> SKMDYDFKVKLSSERERVEDLFEYEGCKVGRGTYGHVYKAKRKDGKDDKDYALKQIEGTGISMSACREIALLRELKHPNVISLQKVFLSHADRKVWLLFDYAEHDLWHIIKFHRASKANKKPVQLPRGMVKSLLYQILDGIHYLHANWVLHRDLKPANILVMGEGPERGRVKIADMGFARLFNSPLKPLADLDPVVVTFWYRAPELLLGARHYTKAIDIWAIGCIFAELLTSEPIFHCRQEDIKTSNPYHHDQLDRIFNVMGFPADKDWEDIKKMPEHSTLMKDFRRNTYTNCSLIKYMEKHKVKPDSKAFHLLQKLLTMDPIKRITSEQAMQDPYFLEDPLPTSDVFAGCQIPYPKREFLTEEEPDDKGDK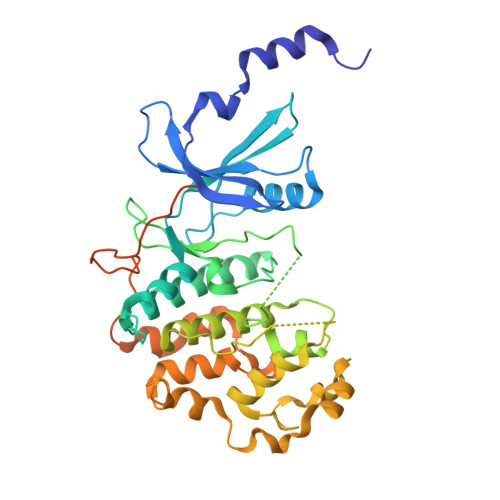KNQQQQQGNNHTNGTGHPGNQDSSHTQGPPLKK> QAQITGRPEWIWLALGTALMGLGTLYFLVKGMGVSDPDAKKFYAITTLVPAIAFTMYLSMLLGYGLTMVPFGGE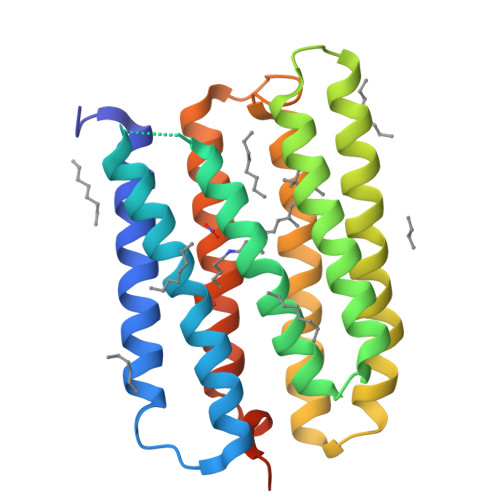QNPIYWARYASWLFTTPLLLLDLALLVDADQGTILALVGADGIMIGTGLVGALTKVYSYRFVWWAISTAAMLYILYVLFFGFTSKAESMRPEVASTFKVLRNVTVVLWSAYPVVWLIGSEGAGIVPLNIETLLFMVLDVSAKVGFGLILLRSRAIFGEAEAPEPSAGDGAAATSD> GUCUACCUAUCGGGCUAAGGAGCCG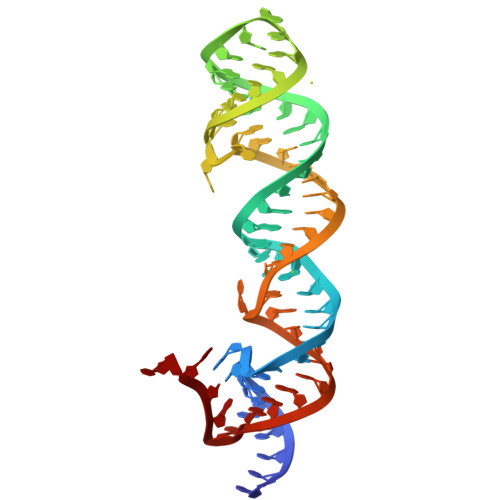UAUGCGAUGAAAGUCGCACGUACGGUUCUAUGCCCGGGGGAAAAC>[2x]SMSGGGEQPDILSVGILVKERWKVLRKIGGGGFGEIYDALDMLTRENVALKVESAQQPKQVLKMEVAVLKKLQGKDHVCRFIGCGRNDRFNYVVMQLQGRNLADLRRSQSRGTFTISTTLRLGRQILESIESIHSVGFLHRDIKPSNFAMGRFPSTCRKCYMLDFGLARQFTNSCGDVRPPRAVAGFRGTVRYASINAHRNREMGRHDDLWSLFYMLVEFVVGQLPWRKIKDK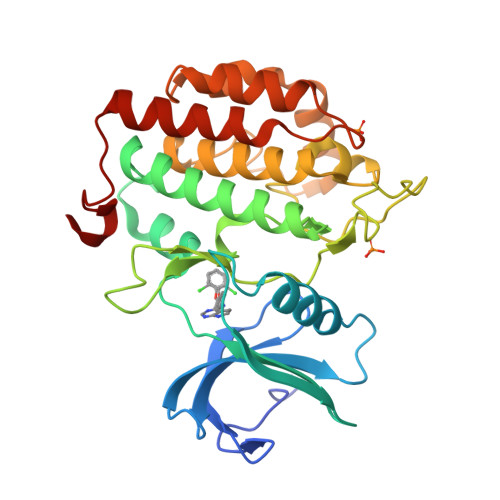EQVGSIKERYDHRLMLKHLPPEFSIFLDHISSLDYFTKPDYQLLTSVFDNSIKTFGVIESDPFDWEK>GPMAINENKKDIKDIVNEILISLNINESINIEIKPMKQKIASFSFKTKTLRLNKYVVENFDEELLHYIILHELIHFKIKSI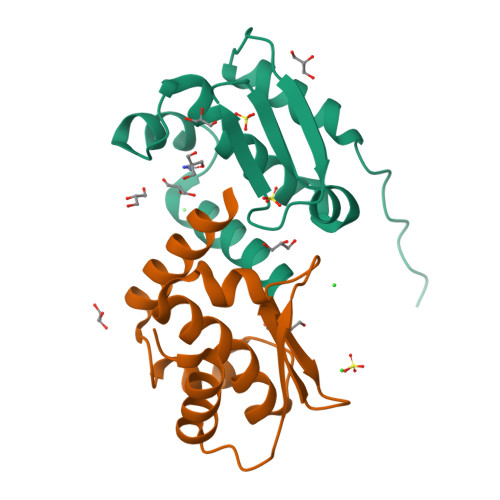NHGIKFENELRNYFSKNECDEIELKIIQKLI[2x]>SSHHHHHHMSGENLYFQGASAAIVTDTGGVDDKSFNQSAWEGLQAWGKEHNLSKDNGFTYFQSTSEADYANNLQQAAGSYNLIFGVGFALNNAVKDAAKEHTDLNYVLIDDVIKDQKNVASVTFADNESGYLAGVAAAKTTKTKQVGFVGGIESEVISRFEAGFKAGVASVDPSIKVQVDYAGSFGDAAKGKTIAAAQYAAGADIVYQVAGGTGAGVFAEAKSLNESRPENEKVWVIGVDRDQEAEG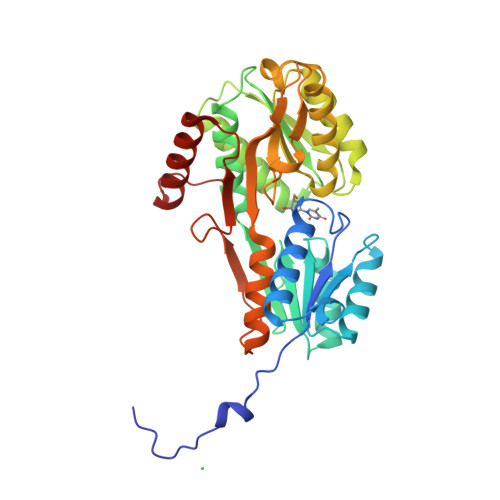KYTSKDGKESNFVLVSTLKQVGTTVKDISNKAERGEFPGGQVIVYSLKDKGVDLAVTNLSEEGKKAVEDAKAKILDGSVKVPE[4x]>MTKENICIVFGGKSAEHEVSILTAQNVLNAIDKDKYHVDIIYITNDGDWRKQNNITAEIKSTDELHLENGEALEISQLLKESSSGQPYDAVFPLLHGPNGEDGTIQGLFEVLDVPYVGNGVLSAASSMDKLVMKQLFEHRGLPQLPYISFLRSEYEKYEHNILKLVNDKLNYPVFVKPANLGSS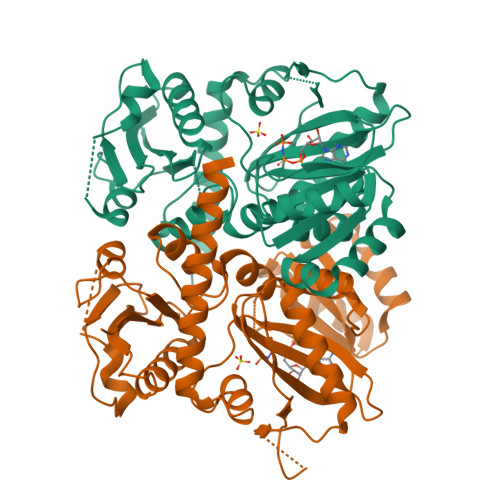VGISKCNNEAELKEGIKEAFQFDRKLVIEQGVNAREIEVAVLGNDYPEATWPGEVVKDVAFYDYKSKYKDGKVQLKIPADLDEDVQLTLRNMALEAFKETDCSGLVRADFFVTEDNQIYINETNAMPGFTAFSMYPKLWENMGLSYPELITKLIELAKERHQDKQKNKYKIDLEHHHHHH[2x]> MPVLNLNDPQAVERYEEFMRQSPYGQVTQDLGWAKVKNNWEPVDVYLEDDQGAIIAAMSMLLGDTPTDKKFAYASKGPVMDVTDVDLLDRLVDEAVKALDGRAYVLRFDPEVAYSDEFNTTLQDHGYVTRNRNVADA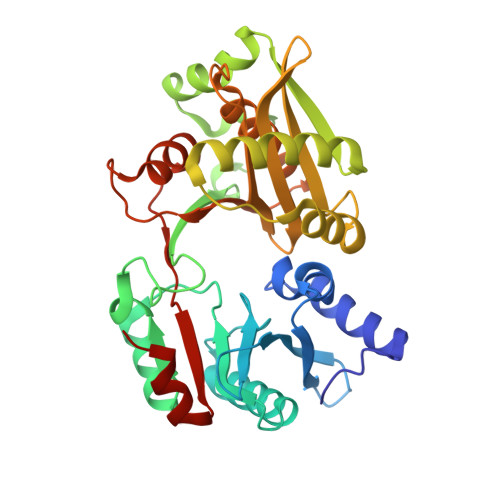GMHATIQPRLNMVLDLTKFPDAKTTLDLYPSKTKSKIKRPFRDGVEVHSGNSATELDEFFKTYTTMAERHGITHRPIEYFQRMQAAFDADTMRIFVAEREGKLLSTGIALKYGRKIWYMYAGSMDGNTYYAPYAVQSEMIQWALDTNTDLYDLGGIESESTDDSLYVFKHVFVKDAPREYIGEIDKVLDPEVYAELVKD>QENSFTINSVDMKSLPDWTVQNGKQLTLQCFADVSTTSHVKPQHQMLFYKDDVLFYQISSMKSTESYFIPEVRIYDSGTYKCTVIVNNKEKTTAEYQLLVEGVPSPRVTLDKKEAIQGGIVRVQCSVPEEKAPIHFTIEKLELNEKMVKLKREKNSRDQNFVILEFPVEEQDRVLSFRCQARIISGIHMQTSESTKSELVTVTESTGHHHHHH[2x]

Platelet–endothelial-cell adhesion molecule-1 (PECAM-1), also well known as CD31, is a 130 kilodalton protein which belongs to both type I transmembrane glycoprotein and immunoglobulin (Ig) superfamily. PECAM-1 can be divided into three parts: extracellular region which contains six immunoglobulin-like (IgL) domains with nine potential N-glycosylation sites, transmembrane region with one single α helix, and cytoplasmic region which possesses two separate tyrosine residues (Y663 and Y686) described as immunoreceptor tyrosine-based inhibitory motifs (ITIMs). As a cell adhesion molecule, PECAM-1 functions principally in cell junction but also plays a role in leukocyte trafficking and immune response. Among adjacent endothelial cells, PECAM-1 interacts with homogeneous molecules in a trans-homophilic binding manner that does not rely on transmembrane and cytoplasmic regions.

To avoid the uncontrolled glycosylation in insect cell expression system that might impair crystallization, we mutated three potential glyco-sites on IgL1-2 (N52Q, N84Q and N151Q). The whole structure of IgL1-2 was finally determined to 3.0 Å resolution where one asymmetric unit contains two IgL1-2 molecules (chains A and B) forming a dimer. The homodimer of PECAM-1 IgL1-2 displays a trans-binding pattern that relies on the interactions between IgL1 and IgL2 derived from two opposite molecules. The two IgL1-2 fragments are packed to each other in a face-to-face antiparallel pattern with the side face of one β sheet. There are two interacting surfaces, one between IgL1 of chain A (IgL1-A) and IgL2 of chain B (IgL2-B) and the other between IgL2 of chain A (IgL2-A) and IgL1 of chain B (IgL1-B). After analyzing the interaction surface of IgL1-2 dimer, the solvent accessible areas buried in interfaces on chain A and B are 1079.0 Å2 and 1094.2 Å2 respectively, and there are two types of reciprocities consisting of hydrophobic interaction and hydrogen bond. On interface1 (IgL2-A-IgL1-B), residues including K158, N187, F188 from IgL2-A and L74, L81, E117 from IgL1-B form the core of the hydrophobic interactions, while N115 from IgL1-B forms satellite hydrophobic interactions with I190, R149 from IgL2-A by donating C and O atoms on backbone to reinforce the hydrophobic contact. Similarly, interface2 (IgL1A-IgL2-B) residues including L74, I112, K116 from IgL1-A and R149, P155, F188, I190 from IgL2-B form the hydrophobic center while the C/O atoms from N115, Q84 on IgL2-A and N187 on IgL1-B form satellite hydrophobic interactions. Thus, the hydrophobic binding core surrounded by hydrogen bonds gives rise to the homophilic dimerization of IgL1-2. No interface was found in one asymmetric unit except the “bridge” contact. In contrast, our structure shows trans-homophilic dimerization of native IgL1-2 in one asymmetric unit, and the last peptide chain 214–228 in IgL2 does not swing out from its own architecture (Sup Fig. 3).>MVMDRPVIVALDLDNEEQLNKILSKLGDPHDVFVKVGMELFYNAGIDVIKKLTQQGYKIFLDLKMHDIPNTVYNGAKALAKLGITFTTVHALGGSQMIKSAK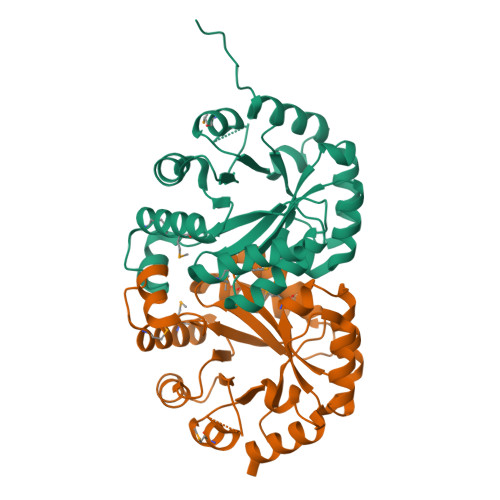DGLIAGTPAGHSVPKLLAVTELTSISDDVLRNEQNCRLPMAEQVLSLAKMAKHSGADGVICSPLEVKKLHENIGDDFLYVTPGIRPAGNAKDDQSRVATPKMAKEWGSSAIVVGRPITLASDPKAAYEAIKKEFNAENLYFQSHHHHHHWSHPQFEK[2x]>TRDQNGTWEMESNENFEGYMKALDIDFATRKIAVRLTQTKVI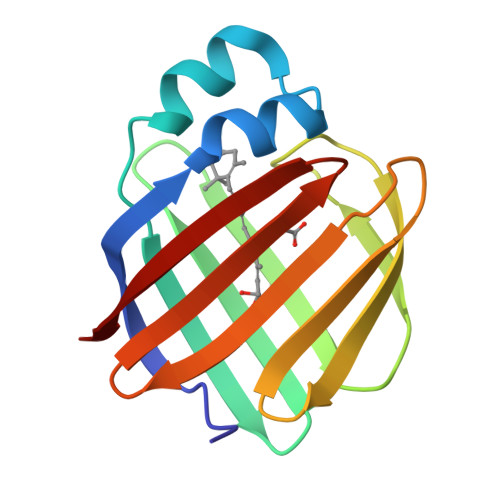DQDGDNFKTKTTSTFRNYDVDFTVGVEFDEYTKSLDNRHVKALVTWEGDVLVCVQKGEKENRGWKQWIEGDKLYLELTCGDQVCRQVFKKK[4x]>[6x]GGGGGGMADLFSTVQEKVAGKDVKIVFPEGLDERILEAVSKLAGNKVLNPIVIGNENEIQAKAKELNLT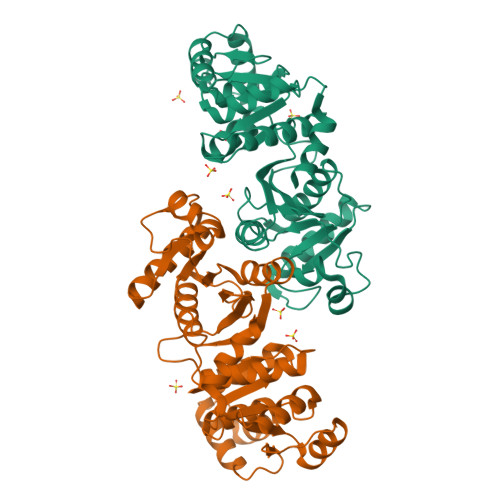LGGVKIYDPHTYEGMEDLVQAFVERRKGKATEEQARKALLDENYFGTMLVYKGLADGLVSGAAHSTADTVRPALQIIKTKEGVKKTSGVFIMARGEEQYVFADCAINIAPDSQDLAEIAIESANTAKMFDIEPRVAMLSFSTKGSAKSDETEKVADAVKIAKEKAPELTLDGEFQFDAAFVPSVAEKKAPDSEIKGDANVFVFPSLEAGNIGYKIAQRLGNFEAVGPILQGLNMPVNDLSRGCNAEDVYNLALITAAQAL>MNNDNPLFKSAMVALSLKISIGNVVKTMQFEPSTMVYDACRMIRERIPEALAGPPNDFGLFLSDDDPKKGIWLEAGK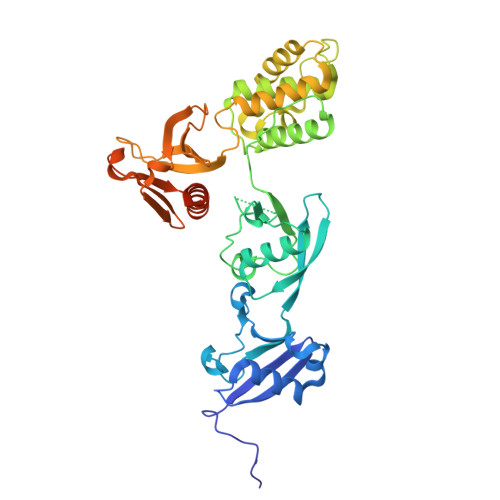ALDYYMLRNGDTMEYRKKQRPLKIRMLDGTVKTIMVDDSKTVTDMLMTICARIGITNHDEYSLVRELMEEKKDELNWLDHGRTLREQGVEEHETLLLRRKFFYSDQNVDSRDPVQLNLLYVQARDDILNGSHPVSFDKACEFAGFQCQIQFGPHNEQKHKAGFLDLKDFLPKEYVKQKGERKIFQAHKNCGQMSEIEAKVRYVKLARSLKTYGVSFFLVKEKMKGKNKLVPRLLGITKECVMRVDEKTKEVIQEWSLTNIKRWAASPKSFTLDFGDYQDGYYSVQTTEGEQIAQLIAGYIDIILKKKKSKDHFGLEGDEESTMLEDSVSPKKST[2x]> MSKVTLNGQQIDF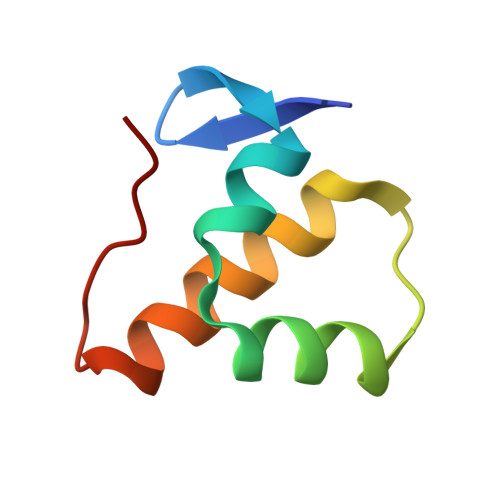DAAVNLMDAELREELHSAQEWTNDQEFLDAYVQAHAAKFDGEEFQVA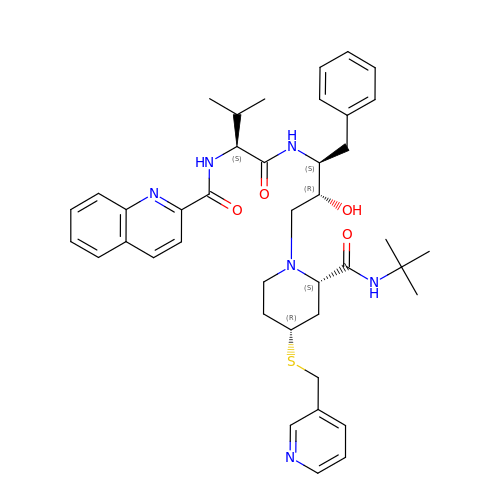N-[(1R)-1-{[(1S,2S)-1-benzyl-3-{(2R,4S)-2-(tert-butylcarbamoyl)-4-[(pyridin-3-ylmethyl)sulfanyl]piperidin-1-yl}-2-hydroxypropyl]carbamoyl}-2-methylpropyl]quinoline-2-carboxamide | C41 H52 N6 O4 S | IMPWGYVYFQPDFN-SZNOJMITSA-N dotinurad | C14 H9 Cl2 N O4 S | 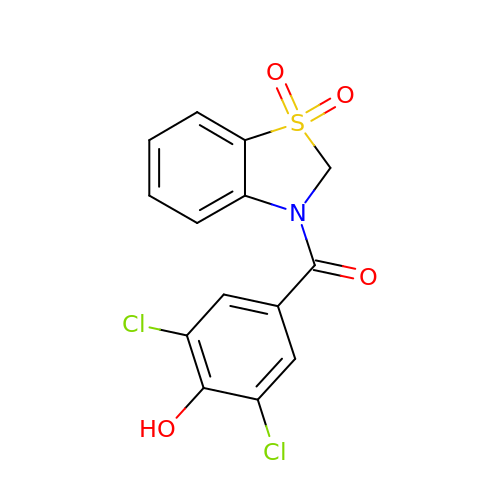VOFLAIHEELWYGO-UHFFFAOYSA-N SAH, which is formed upon methyl-group transfer from SAM, must be removed from the reaction equilibrium (which is shifted far towards SAH formation) by its hydrolase (SAHase; De La Haba & Cantoni, 1959), which splits it into Ado and homocysteine (Hcy). In this way, SAHase is a key regulator of SAM-dependent methylation reactions and of Hcy levels, which, when elevated, are a risk factor for neurodegenerative diseases, neural tube defects and cardiovascular diseases. A typical SAHase protomer is usually divided into three closely connected domains: an N-terminal substrate-binding domain, a cofactor-binding domain and a small C-terminal dimerization domain. The substrate-binding and cofactor-binding domains are separated by a bipartite hinge, allowing them to oscillate between two conformational states, closed and open, during the catalytic cycle.

The structure of BeSAHase in the crystal obtained by cocrystallization with cordycepin of a protein sample that had not been treated with ammonium sulfate (see §2.2.1) is a tetramer with three sub­units (A, B and C) complexed with Ado molecules and one subunit (D) with Cord bound in the active site. One NAD+ molecule is clearly defined by electron density in each subunit. There are three sodium cations near the active site of subunits A, B and C. 1490 water molecules plus three PEG molecules and one acetate ion from the crystallization buffer were located in the solvent region. The Ado molecules in structure (i) were sequestered by the protein during overexpression in E. coli cells. Since the protein:cordycepin molar ratio was 1:8 and the original Ado ligand was apparently replaced in only 25% of the cases, this may suggest that the affinity of BeSAHase for cordycepin is over an order of magnitude lower than that for adenosine, leading to the conclusion that cordycepin would not be a good candidate as an inhibitor of SAHase. The most interesting situation is found in subunit D of the Ado/Cord complex, where cordycepin is bound. When cordycepin is bound in the active site, the protein molecule assumes a semi-open conformation that is intermediate between the canonical open and closed states. The backbone conformation of subunit D is sufficiently different (see §3.3) as to place the side chain of Glu197 in a different direction, so that the hydrogen bond between the O2′ atom of cordycepin and Glu197 O∊2 cannot be formed (the distance between these atoms is 4.1 Å). Also, the hydrogen bonds created with the participation of the O5′ atom are not observed in chain D of the Ado/Cord complex , because the γ torsion angle (defined by the O5′—C5′—C4′—C3′ atoms of the ribose moiety) of the cordycepin ligand is twisted by ∼100° with respect to that of the Ado molecules.

>[4x]GIDPFTMNAKPGFTDYIVKDIALADFGRKEISLAETEMPGLMATREEYGPKQPLKGARIAGSLHMTIQTAVLIETLAALGADIRWVSCNIYSTQDHAAAAIAAAGIPVFAVKGETLTEYWDYTAKLFDWHGGGTPNMILDDGGDATMLVHAGYRAEQGDTAFLDKPGSEEEEIFYALVKRLLKEKPKGWFAEIAKNIKGVSEETTTGVHRLYEMANKGTLLFPAINVNDSVTKSKFDNLYGCRESLVDGIRRGTDVMLSGKVAMVAGFGDVGKGSAASLRQAGCRVMVSEVDPICALQAAMEGYEVVTMEDAAPRADIFVTATGNKDIITIEHMRAMKDRAIVCNIGHFDNEIQIASLRNLKWTNIKPQVDEIEFPDKHRIIMLSEGRLVNLGNAMGHPSFVMSASFTNQTLAQIELFANNKDSKYAKKVYVLPKTLDEKVARLHLAKIGVKLTELRKDQADYIGVKQEGPYKSDHYRY> GDITHMEKLGDICFSLRYVPTAGKLTVVILEAKNLKKMGVGGLSDPYVKIHLMQNGKRLKKKKTTIKKNTLNPYYNESFSFEVPFEQIQKVQVVVTVLDYDKI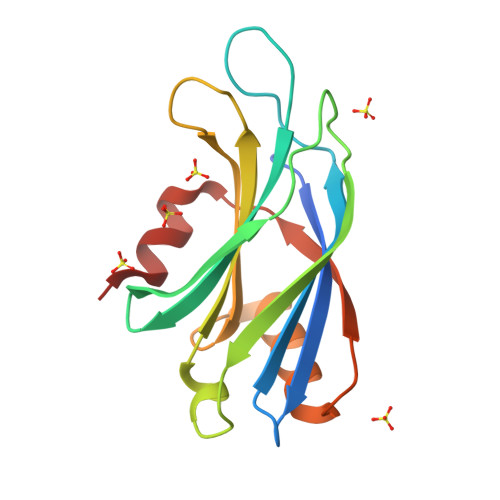GKNDAIGKVFVGYNSTGAELRHWSDMLANPRRPIAQWHTLQVEEEVDAMLAVKK>NSLPYGKINGTYKGTEKEKIKFSSEGSFDPDGKIVSYEWDFGDGNKSNEENPEHSYDKVGTYTVKLK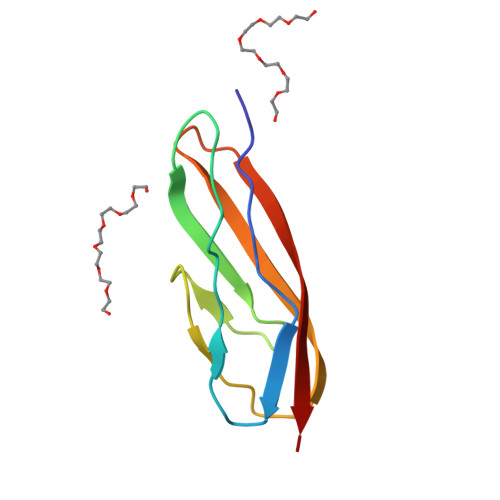VTDDKGESSVSTTTAEIKD[4x]(~{E})-~{N}-[(2~{S},3~{R})-1,3-bis(oxidanyl)octadecan-2-yl]octadec-9-enamide | C36 H71 N O3 | 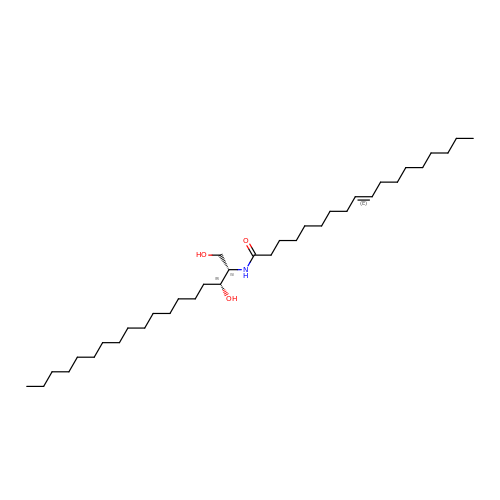MJQIARGPQMNBGT-CJDDIQBSSA-N>[4x]HHHHHHSSGLVPRGSHMVKIGINGFGRIGRLVFRASLERTDVEVVAI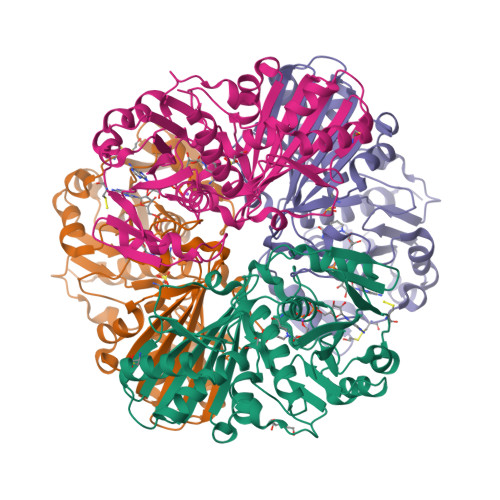NDIMMTPEYMIYMIKYDTVHGKFHGKLEHTEKSIIVNGREIHVLCERDPEQLPWGQHNVEYVVESTGIFTKLDSAAKHLKGGAKRVVISAPADTPTFVMGVNNHEYKPEMTVINNASCTTNCLAPIAAVLHENFGIVEGLMTTVHAVTATQPTVDAPSRKDWRGGRAAGYNIIPSSTGAAKAVGLVIPSLNGKLTGMAFRVPTVDVSVVDLTCRLEKPATKKQIDEAMKAASESERFKGILKFTDEEVVSSDFVHDSASSTYDSKASICLNEHFVKVVAWYDNEWGYSNRVLDLIKSTAKIQ[(2R,5S)-2,5-dimethylmorpholin-4-yl](1,2,5-thiadiazol-3-yl)methanone 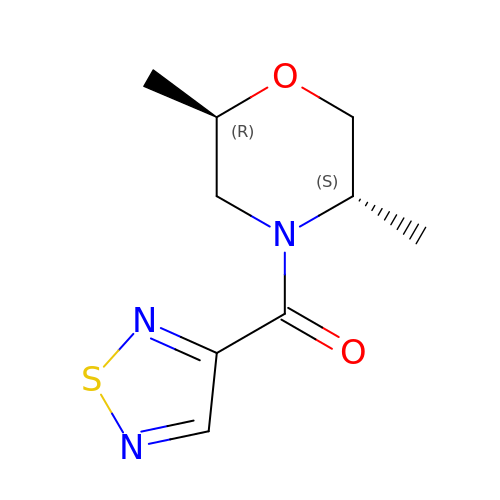| C9 H13 N3 O2 S | IKMQGCCZPWFVJE-NKWVEPMBSA-N>KPIEIIGAPFSKGQPRGGVEKGPAALRKAGLVEKLKETEYNVRDHGDLAFVDVPNDSPFQIVKNPRSVGKANEQLAAVVAETQKNGTISVVLGGDHSMAIGSISGHARVHPDLC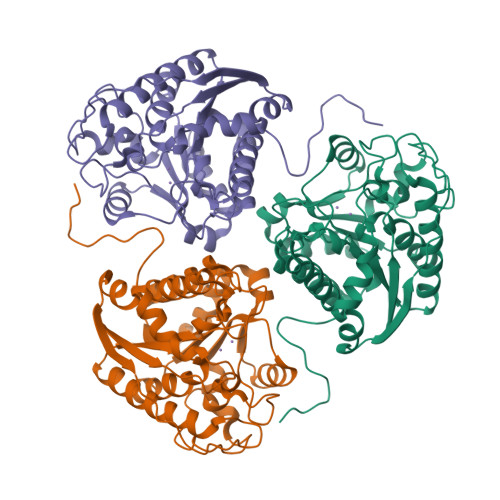VIWVDAHTEINTPLTTSSGNLHGQPVAFLLKELKGKFPDVPGFSWVTPCISAKDIVYIGLRDVDPGEHYIIKTLGIKYFSMTEVDKLGIGKVMEETFSYLLGRKKRPIHLSFDVDGLDPVFTPATGTPVVGGLSYREGLYITEEIYKTGLLSGLDIMEVNPTLGKTPEEVTRTVNTAVALTLSCFGTKREGNHKPETDYL[3x]>GSHMISNDAIRRNMAVFSMSVVSKLTDLTPRQIRYYETHELIKPERTEGQKRLFSLNDLERLLEIKSLLEKGFNIKEIKQII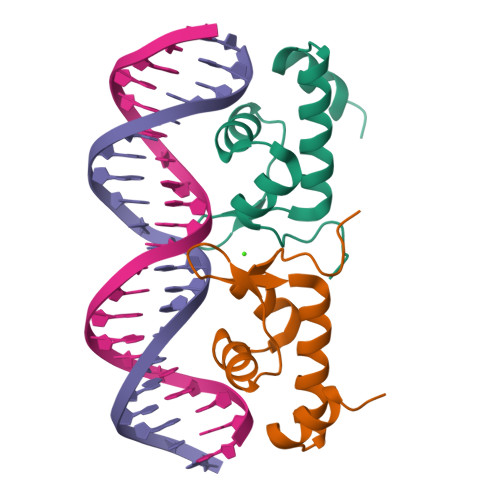YDSQ[4x]> GSTGGVQTVTLIPGDGIGPEISAAVMKIFDAAKAPIQWEERNVTAIQGPGGKWMIPSEAKESMDKNKMGLKGPLKTPIAAGHPSMNLLLRKTFDLYANVRPCVSIEGYKTPYTDVNIVTIRENTEGEYSGIEHVIVDGVVQSIKLITEGASKRIAEF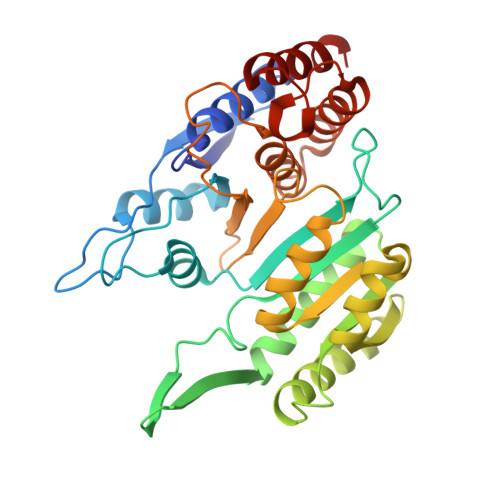AFEYARNNHRSNVTAVHKANIMRMSDGLFLQKCREVAESCKDIKFNEMYLDTVCLNMVQDPSQFDVLVMPNLYGDILSDLCAGLIGGLGVTPSGNIGANGVAIFESVHGTAPDIAGKDMANPTALLLSAVMMLRHMGLFDHAARIEAACFATIKDGKSLTKDLGGNAKCSDFTEEICRRVKDLD>[16x]HHHHHHMRLKIAKESLLNVLSHVVGAVERRHTLNILSNVKIQTNAQALTITGSDLEVELVASTALSEGACLEAGETTVPARKLMEICKSLPTAALIDLQITEDQRCILKSGNSRFVLGTLPAEDYPLLTTENSQGTQVQVTQRELKRLFEKTAFAMAVQDVRFYLTGTLLEIDENQLRAVTT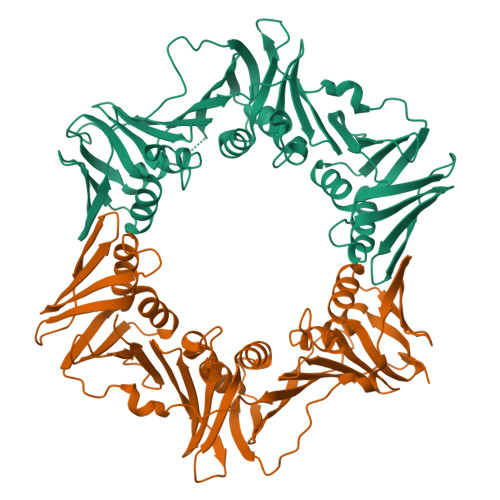DGHRLALCEILASSTSSQLVQAIVPRKAVGELQRLLSIEDEQLTLLIGRELLNVTINTPSRDKEQGDITVRFTTKLIDGKFPDYRRVIPRGGDKHVLIGHDVFKQSLQRVAILSNEKLRGVFLNFNQDSLQLRANNPEQDEAIEDLAIQYQSAPLEMSFNAQYLLDVLGVLDGDDVNMSMTEANQSVLVQDPAHPDQTYVVMPMRV> NGYENP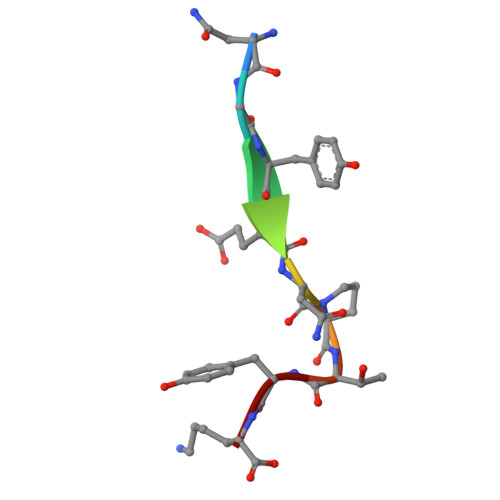TYK>SMAKRVFFSFHYQDVIDFRVNVVRNHWVTKLNQSAAGVFDASLWEDAKKTSDIALKRLINGGLNNTSVTCVLIGSQTFNRRWVRYEIMKSIEKGNKIIGIHINAFKDKYGNIKSKGPNPFDYLGYQYSSDGKQLHLYEWTGGKWEEYKDLAPYRVNQIAPESLRGKFYSLSSVYRVYDWVADDGYNKFSSWVN[2x];>[2x]MNSITHAEFEFSLLENVKYETEDEVPIVLEYKEEIINLIKKFSNSGQSGMSAPITASIITNCIKNLMAFKPIGPLVGNEEEWNYNSDDSFQNNRLSAVFKTGLN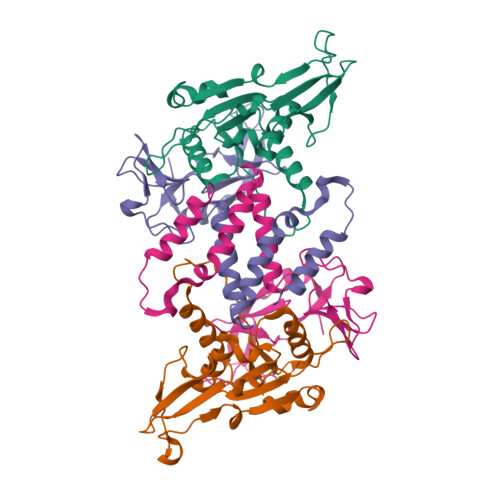GKPYYLDAITFVGEEEYDTFHGHVEGISSRQYLKGFPFFPKTFYINVYKDFENKDENNLCSGDDGEYTYRIKYPEQLEEVFNYYDKFTKE>GSHTAEEDMED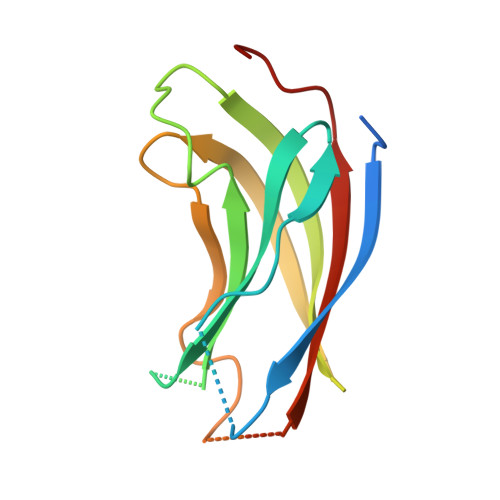DTSWRSEATFQFTVERFSRLSESVLSPPCFVRNLPWKIMVMPRFYPDRPHQKSVGFFLQCNAESDSTSWSCHAQAVLKIINYRDDEKSFSRRISHLFFHKENDWGFSNFMAWSEVTDPEKGFIDDDKVTFEVFVQADAPHGVAW[3x]Pteridine reductase 1 (PTR1) is a key enzyme of the folate pathway in protozoan parasites of the genera Leishmania and Trypanosoma and is a valuable drug target for tropical diseases. This enzyme is able to catalyze the NADPH-dependent reduction of both conjugated (folate) and unconjugated (biopterin) pterins to their tetrahydro forms, starting from oxidized- or dihydro-state substrates. Contiguous to the substrate-binding pocket, a triad of residues, Asp181–Tyr194–Lys198, form a hydrogen-bond network which has been reported to be crucial for the catalytic process.

We determined the crystal structure of LmPTR1 in complex with folate at 1.81 Å resolution in the orthorhombic space group P212121. The PTR1 macromolecule shows the characteristic homotetramer with 222 point-group symmetry and can be directly compared with all of the available structures reported in the literature. The binding mode of FOL is mainly driven by an aromatic stacking interaction between the bicyclic pterin moiety, the Phe113 side chain and the NADP(H) nicotinamide. All of the functional groups of the FOL pteridine core participate in hydrogen-bonding interactions with the enzyme. The FOL amino group at position 2 is hydrogen-bonded to the Ser111 side-chain hydroxyl (2.8–2.9 Å), the carbonyl at position 4 of the FOL molecule is able to establish water-mediated interactions with the side chain of Arg17, and the N atom at position 8 is within hydrogen-bonding distance of the hydroxyl group of Tyr194 of the catalytic triad (2.7–2.8 Å). The terminal glutamate (Glu) tail of folate has been modeled in multiple conformations: in one conformation the Glu tail is oriented towards the β4–α4 loop, while in the other conformation it is placed towards the β6–α7 loop. As a consequence, it may be possible that in our structure the folate is oriented in the active pocket to receive the hydride from the cofactor but the Asp is not yet protonated and still unable to start the catalytic process. Indeed, the L. major and T. brucei enzymes appear to be 2/4-fold (LmPTR1) to tenfold (TbPTR1) faster in reducing unconjugated pterins than folate. It may be conceivable that the slower kinetics shown by both LmPTR1 and TbPTR1 in reducing folate compared with unconjugated substrates has allowed the initial binding of a folate molecule to the enzyme to be trapped in our crystal structure before the beginning of the catalytic process.

>[4x]MTAPTVPVALVTGAAKRLGRSIAEGLHAEGYAVCLHYHRSAAEANALSATLNARRPNSAITVQADLSNVATAPVSGADGSAPVTLFTRCAELVAACYTHWGRCDVLVNNASSFYPTPLLRNDEDGHEPCVGDREAMETATADLFGSNAIAPYFLIKAFAHRVAGTPAKHRGTNYSIINMVDAMTNQPLLGYTIYTMAKGALEGLTRSAALELAPLQIRVNGVGPGLSVLVDDMPPAVWEGHRSKVPLYQRDSSAAEVSDVVIFLCSSKAKYITGTCVKVDGGYSLTRA> LPTLGPGWQRQNPDPPVSRTRSLLLDAASGQLRLEDGFHPDAVAWANLTNAIRETGWAYLDLSTNGRYNDSLQAYAAGVVEASVSEELIYMHWMNTVVNYCGPFEYEVGYCEKLKNFLEANLEWMQREMELNPDSPYWHQVRLTLLQLKGLEDSYEGRLTFPTGRFTIKPLGFLLLQISGDLEDLEPALNKTNTKPSLGSGSCSALIKLLPGGHDLLVAHNTWNSYQNMLRIIKKYRLQFREGPQEEYPLVAGNNLVFSSYPGTIFSGDDFYILGSGLVTLETTIGNKNPALWKYVQPQGCVLEWIRNVVANRLALDGATWADVFKRFNSGTYNNQWMIVDYKAFLPNGPSPGSRVLTILEQIPGMVVVADKTAELYKTTYWASYNIPYFETVFNASGLQALVAQYGDWFSYTKNPRAKIFQRDQSLVEDMDAMVRLMRYNDFLHDPLSLCEACNPKPNAENAISARSDLNPANGSYPFQALHQRAHG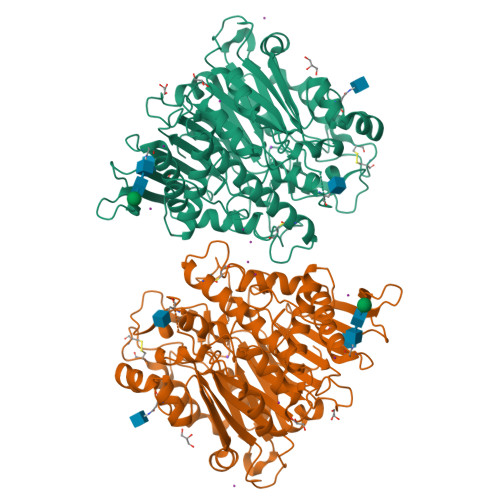GIDVKVTSFTLAKYMSMLAASGPTWDQCPPFQWSKSPFHSMLHMGQPDLWMFSPIRVPWDGRGSHHHHHHG>[2x]MCGIFAYLNYHVPRTRREILETLIKGLQRLEYRGYDSAGVGFDGGNDKDWEANACKIQLIKKKGKVKALDEEVHKQQDMDLDIEFDVHLGIAHTRWATHGEPSPVNSHPQRSDKNNEFIVIHNGIITNYKDLKKFLESKGYDFESETDTETIAKLVKYMYDNRESQDTSFTTLVERVIQQLEGAFALVFKSVHFPGQAVGTRRGSPLLIGVRSEHKLSTDHIPILYRTGKDKKGSCNLSRVDSTTCLFPVEEKAVEYYFASDASAVIEHTNRVIFLEDDDVAAVVDGRLSIHRIKRTAGH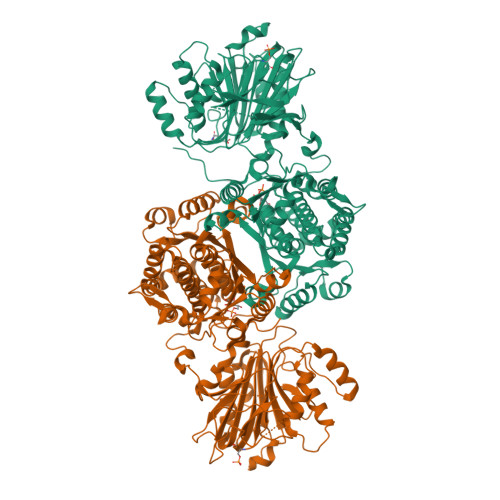HHHHHDHPGRAVQTLQMELQQIMKGNFSSFMQKEIFEQPESVVNTMRGRVNFDDYTVNLGGLKDHIKEIQRCRRLILIACGTSYHAGVATRQVLEELTELPVMVELASDFLDRNTPVFRDDVCFFLSQSGETADTLMGLRYCKERGALTVGITNTVGSSISRETDCGVHINAGPEIGVASTKAYTSQFVSLVMFALMMCDDRISMQERRKEIMLGLKRLPDLIKEVLSMDDEIQKLATELYHQKSVLIMGRGYHYATCLEGALKIKEITYMHSEGILAGELKHGPLALVDKLMPVIMIIMRDHTYAKCQNALQQVVARQGRPVVICDKEDTETIKNTKRTIKVPHSVDCLQGILSVIPLQLLAFHLAVLRGYDVDFPRNLAKSVTVE>CPRFLKVKNWETDVVLTDTLHLKSTLETGCTEHICMGSIVLPSQHTRKPEDVRTKDQLFPLAKEFLDQYYSSIKRFGSKAHMDRLEEVNKEIESTSTYQLKDTELIYGAKHAWRNASRCVGRIQWSKLQVFDARDCTTAHGMFNYICNHVKYATNKGNLRSAITIFPQRTDGKHDFRVWNSQLIRYAGYKQPDGSTLGDPANVQFTEICIQQGWKAPRGRFDVLPLLLQANGNDPELFQIPPELVLEVPIRHPKFDWFKDLGLKWYGLPA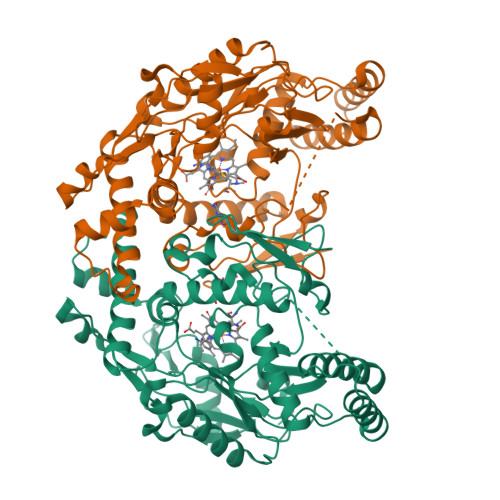VSNMLLEIGGLEFSACPFSGWYMGTEIGVRNYCDNSRYNILEEVAKKMDLDMRKTSSLWKDQALVEINIAVLYSFQSDKVTIVDHHSATESFIKHMENEYRCRGGCPADWVWIVPPMSGSITPVFHQEMLNYRLTPSFEYQPDPWNTHVWKG[2x]> SSSNYCNQMMKSRNLTKDRCKPVNTFVHESLADVQAVCSQKNVACKNGQTNCYQSYSTMSITDCRETGSSKY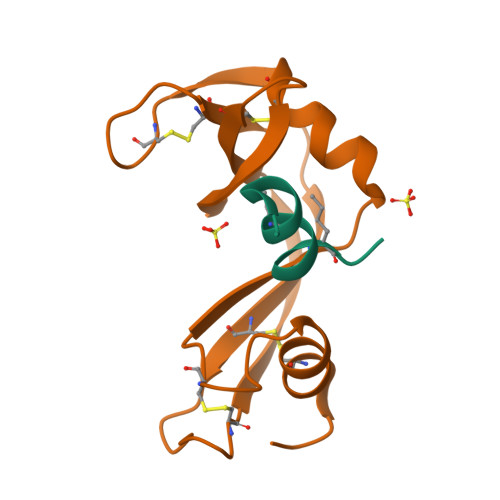PNCAYKTTQANKHIIVACEGNPYVPVHFDASV;> KETAAAKVERQHLDS> M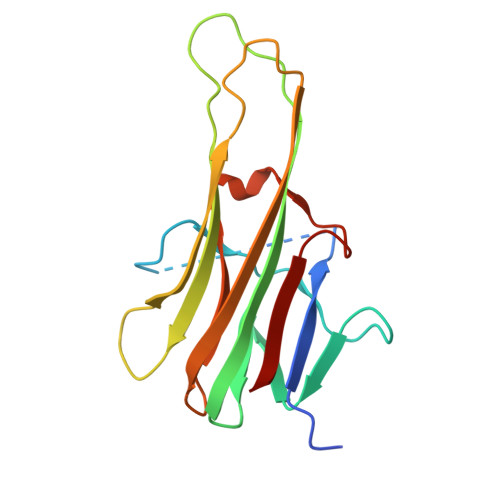VRERGPQRVAAHITGTRGRSNTLSSPNSKNEKALGRKINSWESSRSGHSFLSNLHLRNGELVIHEKGFYYIYSQTYFRFQEEIKENTKNDKQMVQYIYKYTSYPDPILLMKSARNSCWSKDAEYGLYSIYQGGIFELKENDRIFVSVTNEHLIDMDHEASFFGAFLVG> PPGPPEAVTIDEITDTTAQLSWRPGPDNHSPITMYVIQARTPFSVGWQAVNTVPDLVDGKTFTATVVGLNPWVEYEFRTVAANVIGIGEPSRPSEKRRTEEALPEVTPANVSGGGGSKSELVITWETVPEELQNGRGFGYVVAFRPHGKMIWMLTVLASADASRYVFRNESVRPFSPFEVKVGV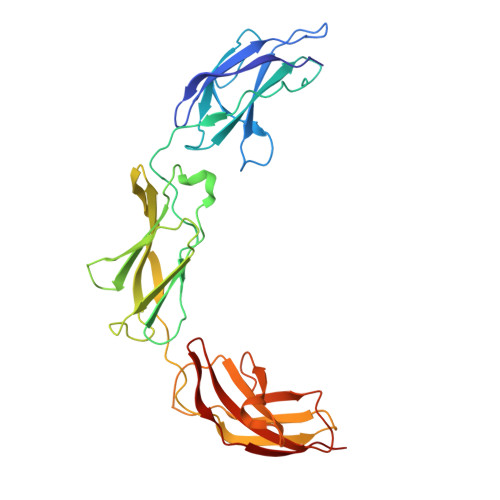FNNKGEGPFSPTTLVYSAEEEPTKPPASIFARSLSATDIEVFWASPIGKNRGRIQGYEVKYWRHDDKEENAKKIRTVGNQTSTKITNLKGSALYHLSVKAYNSAGTGPSSATVNVTTRK1-(3-Chloro-5-trifluoromethoxy-phenyl)-3-[2-(2-hydroxy-ethyl)-phenyl]-urea | C16 H14 Cl F3 N2 O3 | 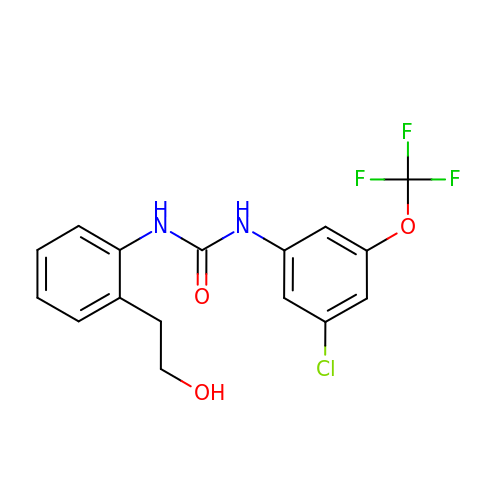MFPOPEHXGDSREH-UHFFFAOYSA-N> MDAPMEDAPAPVAQVKVIFTTTEPDLELPESKRQLLVPADIRRYGLSRILNSESMLDTGSIPFDFLINGSFLRSSLEDYLTSNGLSLETTLTLQYVRSLIPPVYEASFEHDDWVSAVDVLSATSPAGRWSSAANSSAAVQPGQERVLSASYDGLLRIWNASGSVIATSPSGSHGGHTASIKAAKFLTSDRLASAGMDRTVRVWKYTESDHFTGELKPTLELYGHTGSVDWLDVDGHSKHILTASADGAIGFWSASKASAPEPDASLLPGAHVSKRRKATSSVSTAQRGPLGLWSIHTAPATAAIFDPRDRTVAYSASQDHTVRTLDLTTGQVVSTLTLTHPLLSLSALTRAGTTSPLLAAGTSARHITMVDPRASSATTSVMTLRGHANKVVSLSPSPENEYSLVSGSHDGTCRVWDLRSVRPATKEEGSLGGVSEPVY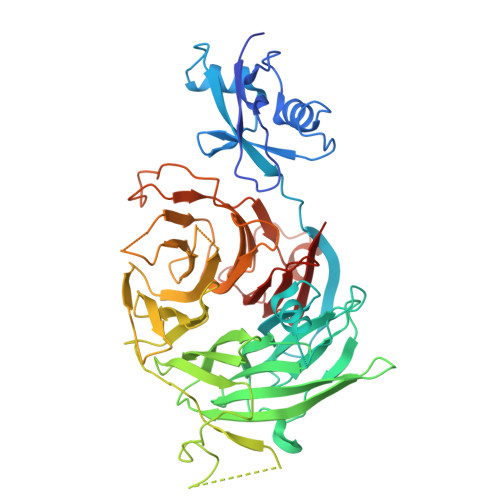VIERESWASKGKKKRPVAGDGCKVFSVVWDKLGIFSGGEDKKVQVNRGRNIVTEQK> MAVEPFPRRPITRPHASIEVDTSGIGGSAGSSEKVFCLIGQAEGGEPNTVYELRNYSQAKRLFRSGELLDAIELAWGSNPNYTAGRILAMRIEDAKPASAEIGGLKITSKIYGNVANNIQVGLEKNTLSDSLRLRVIFQDDRFNEVYDNIGNIFTIKYKGEEANATFSVEHDEETQKASRLVLKVGDQEVKSYDLTGGAYDYTNAIITDINQLPDFEAKLSPFGDKNLESSKLDKIENANIKDKAVYVKAVFGDLEKQTAYNGIVSFEQLNAEGEVPSNVEVEAGEESATVTATSPIKTIEPFELTKLKGGTNGEP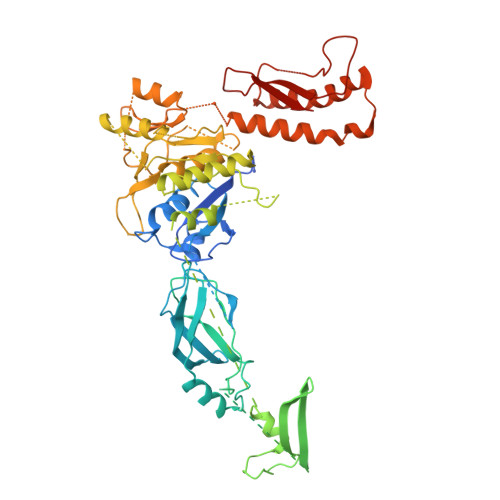PATWADKLDKFAHEGGYYIVPLSSKQSVHAEVASFVKERSDAGEPMRAIVGGGFNESKEQLFGRQASLSNPRVSLVANSGTFVMDDGRKNHVPAYMVAVALGGLASGLEIGESITFKPLRVSSLDQIYESIDLDELNENGIISIEFVRNRTNTFFRIVDDVTTFNDKSDPVKAEMAVGEANDFLVSELKVQLEDQFIGTRTINTSASIIKDFIQSYLGRKKRDNEIQDFPAEDVQVIVEGNEARISMTVYPIRSFKKISVSLVYKQQTLQA>NGEAICSALPTIPYHKLADLRYLSRGASGTVSSARHADWRVQVAVKHLHIHTPLLDSERKDVLREAEILHKARFSYILPILGICNEPEFLGIVTEYMPNGSLNELLHRKTEYPDVAWPLRFRILHEIALGVNYLHNMTPPLLHHDLKTQNILLDNEFHVKIADFGLSKWRMMSLSQSRSSKSAPEGGTIIYMPPENYEPGQKSRASIKHDIYSYAVITWEVLSRKQPFEDVTNPLQIMYSVSQGHRPVINEESLPYDIPHRARMISLIESGWAQN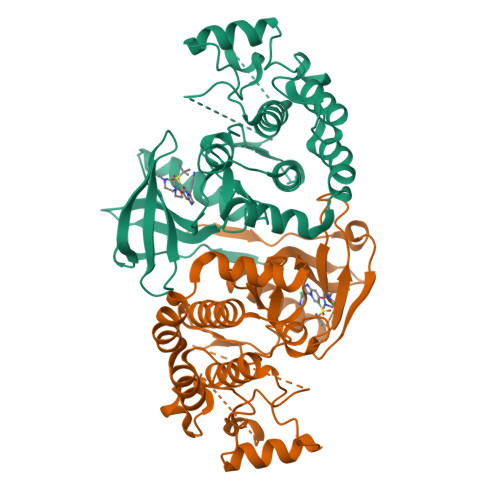PDERPSFLKCLIELEPVLRTFEEITFLEAVIQLKK[16x]> SSSHPIFHRGEFSVCDSVSVWVGDKTTATDI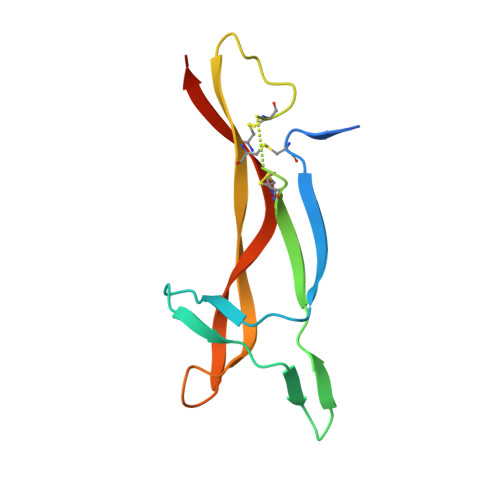KGKEVMVLGEVNINNSVFKQYFFETKCRDPNPVDSGCRGIDSKHWNSYCTTTHTFVKALTMDGKQAAWRFIRIDTACVCVLSRKAVRRA>[4x]MGAMDQEIGTVTDTKMDPRDFLQLLKINAEK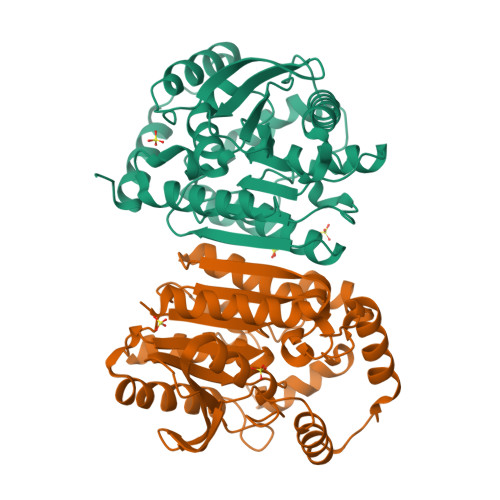AEKNLPLDQKRAGMEALCERFPRAEGVELTLTDLGGVPCIRQATDGAGAAHILYFHGGGYISGSPSTHLVLTTQLAKQSSATLWSLDYRLAPENPFPAAVDDCVAAYRALLKTAGSADRIIIAGDSAGGGLTTASMLKAKEDGLPMPAGLVMLSPFVDLTLSRWSNSNLADRDFLAEPDTLGEMSELYVGGEDRKNPLISPVYADLSGLPEMLIHVGSEEALLSDSTTLAERAGAAGVSVELKIWPDMPHVFQMYGKFVNAADISIKEICHWISARISKLAAALEHHHHHH> MAHHHHHHGTGQDRVVALVDMDCFFVQVEQRQNPHLRNKPCAVVQYKSWKGGGIIAVSYEARAFGVTRSMWADDAKKLCPDLLLAQVRESRGKANLTKYREASVEVMEIMSRFAVIERASIDEAYVDLTSAVQERLQKLQGQPISADLLPSTYIEGLPQGPTTAEETVQKEGMRKQGLFQWLDSLQIDNLTSPDLQLTVGAVIVEEMRAAIERETGFQCSAGISHNKVLAKLACGLNKPNRQTLVSHGSVPQLFSQMPIRKIRSLGGKLGASVIEILGIEYMGELTQFTESQLQSHFGEKNGSWLYAMCRGIEHDPVKPRQLPKTIGCSKNFPGKTALATREQVQWWLLQLAQELEERLTKDRNDNDRVATQLVVSIRVQGDKRLSSLRRCCALTRYDAHKMSHDAFTVIKNCNTSGIQTEWSPPL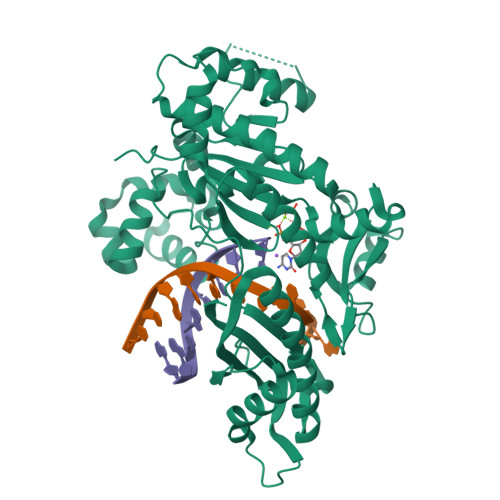TMLFLCATKFSAS To extend the structural coverage of proteins of unknown function, we targeted Pfam protein family PF06684 (domain of unknown function 1185; DUF1185) and determined the crystal structures of two representative members. Despite lacking any recognizable sequence similarity to other protein families, both proteins show significant structural similarity to proteins with a Bacillus chorismate mutase-like (BCM-like) fold characterized by a β-α-β-α-β-β core that includes a mixed β-sheet (order 1423) with the β4 strand antiparallel to the rest. The biological unit of both proteins is a hexamer and analysis of homologs indicates that the oligomer interface residues are highly conserved. Structural similarities to BCM and genome-context analysis suggest a function in amino-acid synthesis.

The BB2672 gene of Bordetella bronchiseptica, which is a causative agent of infectious bronchitis in domestic mammals, encodes a protein with a molecular weight of 20.9 kDa (residues 1–192) and a calculated isoelectric point of 7.1. The crystal structure of BB2672 was determined to 1.7 Å resolution using the SAD method. The final model included three protomers (residues 2–192 of chain A, residues 1–192 of chain B and residues 2–192 of chain C), two tetraethylene glycol (PEG) molecules, 27 ethylene glycol molecules, four chloride ions and 566 water molecules in the asymmetric unit. BB2672 forms a single domain composed of seven β-strands (β1–β7; residues 6–16, 28–38, 78–85, 118–122, 129–135, 146–150 and 160–168), three α-helices (H1, H3 and H4; residues 50–71, 92–95 and 97–108) and three 310-helices (H2, H5 and H6; residues 73–75, 142–144 and 182–184). BB2672 contains a central five-stranded mixed β-sheet with 12734 topology that packs against helices H1, H3 and H4. Analysis of the BB2672 crystallo­graphic hexamer reveals a trimer of dimers, with two distinct types of dimerization interface created by an extra N-terminal strand and a β-­hairpin insertion between strands β3 and β4 in the core BCM-like fold. The more extensive interface, which is located at the C-terminus, contains a network of histidine and salt-bridged residues that may indicate environmental regulation of hexamer assembly. The smaller interface at the N-terminus could present a potential ligand-binding site for the DUF1185 family, the genetic context of which supports a role in amino-acid metabolism. Proximal to this cavity, a highly con­served cluster of four histidines, His93, His98, His144, His174, is located within hydrogen-bonding distance of residues involved in the formation of intermolecular salt bridges. In SPO0826, most of these regions are disordered, indicating flexibility. This clustering of histidine residues in regions of some conformational variability and the proximity of salt bridges involved in oligomerization suggests that assembly of the BB2672 hexamer could be modulated by pH or salt concentration.

>GMSLIEIRKRTLIVETTYHENGPAPAQPLKLAASCAVIRNPYAGRYEPDLMPFMAELRSLGTLLATELVDTLGKDNIEVYSKAAIVGVDGEMEHGAVWHEAGGWAMRSVLGEPKAMVPAVKAVATAGYRMMVPVHYIHASYVRSHFNSIEIGIQDAPRPREILFALVMGTGARVHARLGGLTKEAVSVHDGQR[3x]ATRAZINE GLUTATHIONE CONJUGATE | C18 H30 N8 O6 S | 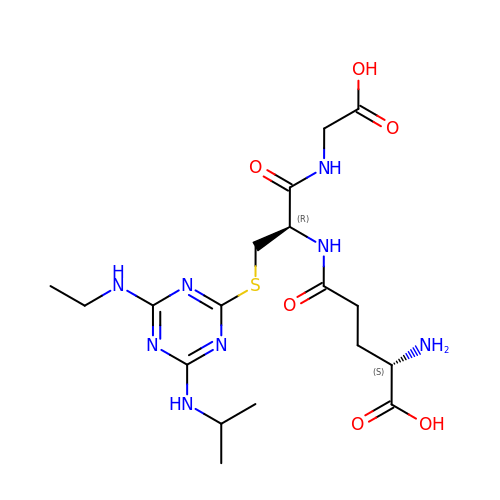WDLCRTLULMGVMR-QWRGUYRKSA-N>[2x]ANDIDNSNPVVQAEQLNWLHYLMNYGSIVANDPEANFDGVRVDAVDNVNADLLQIASDYLKAHYGVDKSEKNAINHLSILEAWSDNDPQYNKDTKGAQLPIDNKLRLSLLYALTRPLEKDASNKNEIRSGLEPVITNSLNNRSAEGKNSERMANYIFIRAHDSEVQTVIAKIIKAQINPKTDGLTFTLDELKQAFKIYNEDMRQAKKKYTQSNIPTAYALMLSNKDSITRLYYGDMYSDDGQYMATKSPYYDAIDTLLKARIKYAAGGQDMKITYVEGDKSHMDWDYTGVLTSVRYGTGANEATDQGSEATKTQGMAVITSNNPSLKLNQNDKVIVNMGTAHKNQEYRPLLLTTKDGLTSYTSDAAAKSLYRKTNDKGELVFDASDIQGYLNPQVSGYLAVWVPVGASDNQDVRVAASNKANATGQVYESSSALDSQLIYEGFSNFQDFVTKDSDYTNKKIAQNVQLFKSWGVTSFEMAPQYVSSEDGSFLDSIIQNGYAFEDRYDLAMSKNNKYGSQQDMINAVKALHKSGIQVIADWVPDQIYNLPGKEVVTATRVNDYGEYRKDSEIKNTLYAANTKSNGKDYQAKYGGAFLSELAAKYPSIFNRTQISNGKKIDPSEKITAWKAKYFN

Streptococcus mutans, a known etiological agent in the pathogenesis of dental caries, expresses three genetically distinct types of glucosyltransferases (Gtfs; also known as glucansucrases): GtfB (GTF-I), GtfC (GTF-SI) and GtfD (GTF-S). GtfC synthesizes both soluble and insoluble glucans (α-1,3 and α-1,6 glycosidic linkages), while GtfB and GtfD only synthesize insoluble glucans (mostly α-1,3 linkages) and soluble glucans (mostly α-1,6 linkages), respectively. All three enzymes belong to glycoside hydrolase family 70 (GH70), which cleaves the glycosidic bond between the glucose and fructose moieties in sucrose during catalysis. While fructose is released, the enzymatically produced glucose molecules are sequentially fused into a growing glucan chain and, depending on whether a 1,3- or 1,6-linkage is formed, the resultant product is either an insoluble or a soluble glucan, respectively.

The new structure of the catalytic domain of GtfD affords a structural comparison of the three S. mutans glycosyltransferases. Initially, GtfB-CD, like GtfD-CD, underwent proteolysis during crystallization setups at room temperature, which we only identified after the structures had been resolved since the gels after purification appeared to be satisfactory. Unfortunately, use of the classic protease inhibitors AEBSF and PMSF had no effect on GtfD-CD. When the models were rebuilt after obtaining molecular-replacement solutions using homology models based on the GtfC-CD structure and the GtfB or GtfD sequences, it was clear that GtfD-CD had missing residues; in fact, the final refined structure of GtfD-CD lacked domains B1 and IV. Our current structure of the catalytic domain for GtfD lacks domains B1 and IV (truncated at residue 421 because of proteolysis). Unfortunately, the catalytic domain of GtfD is not complete since crystallization resulted in the structure of a truncated protein lacking approximately 200 N-terminal residues of domain IV. Although GtfD differs markedly in primary structure (52% sequence identity to GtfB and 61% to GtfC), it still has remarkable similarity in its structural elements (the r.m.s.d. to GtfC is 0.69 Å for 3292 of 3959 aligned atoms and the r.m.s.d. to GtfB is 0.69 Å for 3274 of 3962 aligned atoms). GtfD in particular shows several different residues, with one prominent residue (Thr589 in GtfD) being the decider for the type of glucans (soluble or insoluble) that are formed. The truncated model of GtfD-CD is likewise similar, but our attempts to co-crystallize acarbose with GtfD were unsuccessful due to the absence of key binding residues in the abbreviated GtfD (residues 421–1054).> GSHMKNPYSNQIER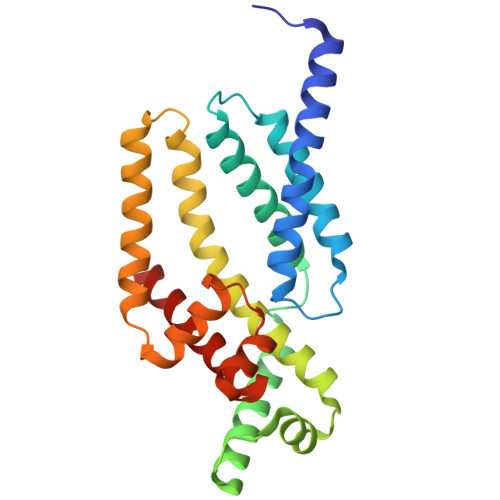EELILKYLPLVKAIATNIKKHLPEDVDIRDLISYGVIGLIKAVDNLSTENPKRAEAYIKLRIKGAIYDYLRSLDFGSRQVREKERRIKEVVEKLKEKLGREPTDEEVAKELGISTEELFKTLDKINFSYILSLEEVFRDFARDYSELIPSSTNVEEEVIKRELTEKVKEAVSKLPEREKLVIQLIFYEELPAKEVAKILETSVSRVSQLKAKALERLREMLSNPL>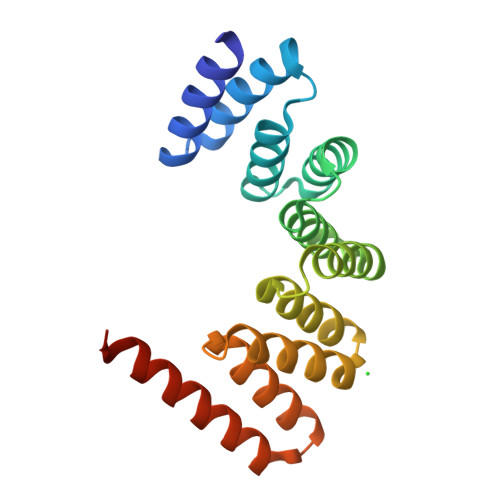[4x]MGETTTIYMDIGDKKRTKGDFDGAIRAYKKVLKADPNNVETLLKLGKTYMDIGLPNDAIESLKKFVVLDTTSAEAYYILGSANFMIDEKQAAIDALQRAIALNTVYADAYYKLGLVYDSMGEHDKAIEAYEKTISIKPGFIRAYQSIGLAYEGKGLRDEAVKYFKKALEKEEKKAKYELALVPR> MQADILDGKQKRVNLNSKRLVNCNQVDVNQLVPIKYKWAWEHYLNGCANNWLPTEIPMGKDIELWKSDRLSEDERRVILLNLGFFSTAESLVGNNIVLAIFKHVTNPEARQYLLRQAFEEAVHTHTFLYICESLGLDEKEIFNAYNERAAIKAK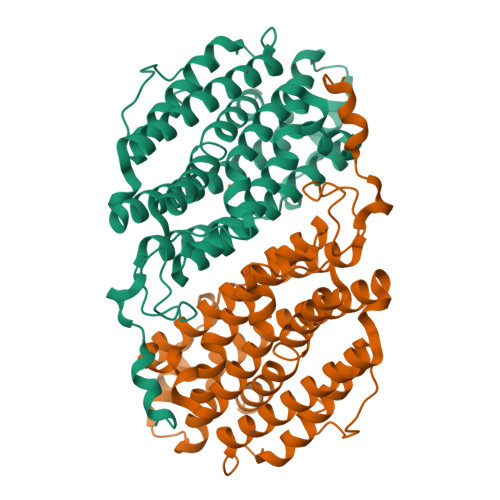DDFQMEITGKVLDPNFRTDSVEGLQEFVKNLVGYYIIMEGIFFYSGFVMILSFHRQNKMIGIGEQYQYILRDETIHLNFGIDLINGIKEENPEIWTPELQQEIVELIKRAVDLEIEYAQDCLPRGILGLRASMFIDYVQHIADRRLERIGLKPIYHTKNPFPWMSETIDLNKEKNFFETRVIEYQHAASLTW> QRRLYDQAKAALAKGNSAPYMASRSALRDYPLEPYLAYDELTHRLKSASNEEVERFLTEHGDLPQIGWLKLRWLRLLADRGDWKTFVNYYDPKLNFTELDCLYGQYQLGHGQKAEGYATSERLWLVGKSQPAACDTLFGLWQGEGQLTEEKVWKRLKLAAEARNYSLASHLAQRLPTLGNQGALMVSVAQNPAQLSQTGRFSQRDHATADVVGLGLRRLARQDPEKALSLLDYYSSALPFSSDEKVAIAREIGLSLAKRFDPRALPLMTQYDPGLRDNTVTEWRTRLLLRLGRWDEAYALTRKLPQDLAATSRWRYWQARSLQLAQPNSKEPIALYQKLAGERDFYGFLAADRLSVPYKLGNRPAHIDPRVLQRVRNAASTRRAMEFFNRGEVINARREWYHAARLFDRDELIAQARLAYDMQWYFPAIRSISQAQYWDDLDIRFPMAHRATLVREAKNRGLHSSWIFAITRQQSAFMSDARSGVGATGLMQLMPGTAKETSRKFGIPLASTQQLIVPDVNIRLGAAYLSQVHSQFNG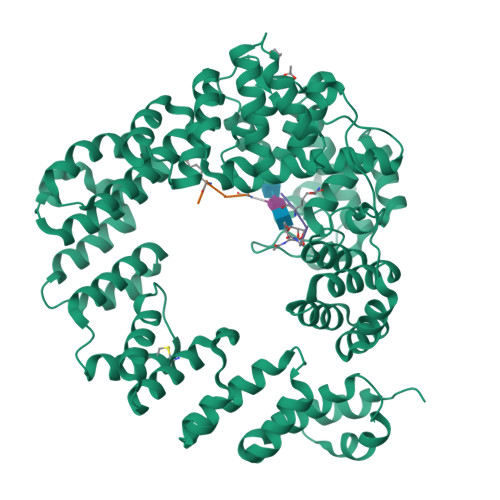NRVLASAAYNAGPGRVRQWLKDTRHLAFDVWIETIPFDETRQYVQNVLSYAVIYGQKLNAPQPIVDWHERYFDDF;>AEKA[2x]>[2x]STTGIIMENVTAFWEEGFGELLEKVQQSNGDRKHSSDENNVSFSHLCLVGNPVLKNINLNIEKGEMLAITGSTGSGKTSLLML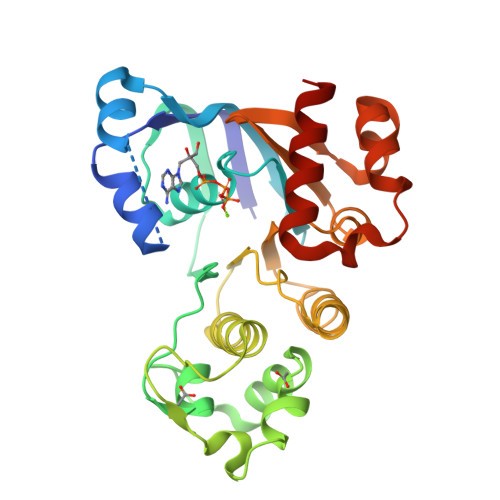ILGELEASEGIIKHSGRVSFCSQFSWIMPGTIKENIIFGVSYDEYRYKSVVKACQLQQDITKFAEQDNTVLGEGGVTLSGGQRARISLARAVYKDADLYLLDSPFGYLDVFTEEQVFESCVCKLMANKTRILVTSKMEHLRKADKILILHQGSSYFYGTFSELQSLRPDFSSKLMGYDTFDQFTEERRSSILTETLRRFSVDD>[2x]GSHMKDYSLEIDAVMKAAQINDTNNFVQALMRWHFSKET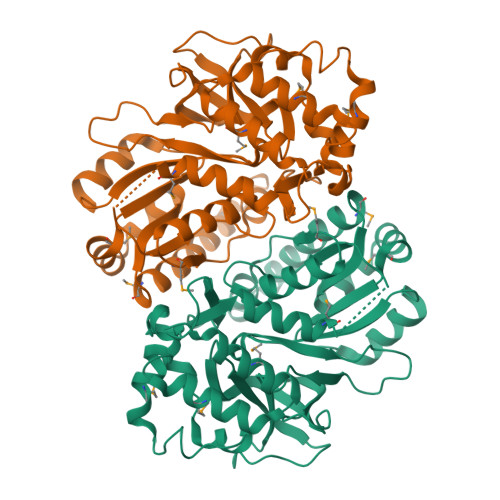GSPFWLGMREQLNFDPIKDVKTINDLRQFSDISHCLRQEPVANLVPQGLPADSHPQVYESGGTTGAPKYVVAYDAWIEALISWRMSGYQHRPGRPSGNTLAAIPTGPHIVGAINKERALRLGGMFFSIDIDPRWVKRSLSEGDTATVRKYTHHLVDQVQNTLMNQDIRFLVTTPPVLRELLKRPEVVLQMKQSLAQITLGGTELNLDEIKFIASEILPDCEFSASYGSTSALGVSRSLLITSESQQVIYDSFSPFITYDVVDSITAQTVEYGERGNVIVTHLSPWAFYPRVAERDTAIRLPGVSGFAGDRLADIEPLKISEGRKVIEGVY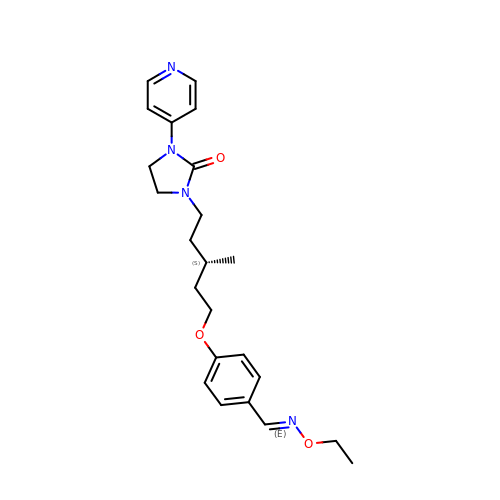1-[(3S)-5-[4-[(E)-ETHOXYIMINOMETHYL]PHENOXY]-3-METHYL-PENTYL]-3-PYRIDIN-4-YL-IMIDAZOLIDIN-2-ONE | C23 H30 N4 O3 | IRYPPICIQPYQGY-YSRPOPIVSA-N>MSGDASSGSPDITGEEQGVAVATGTQPSAPAMATLATAATGTMPEEWKTFFSYYTTVNWSTTDETGKVLFVQGLSPRMNPFLDHLAKMYTGWSGSMEIRFTISGSGVFGGKLAAVMVPPGIGTEGGTSLLQFPHVLVDARQTEPVIFNIPDIRTVLWHDMHDTLTAHLVILVYNDLLNPYQNTTTGTSCTVTVETRGGTDFEFHLLKPPSRKMIFGADPSRLIPKKSMFWEGNRLPGEFKGFSIKPLVFQANRHFDCKRQTFGWSTPEHAGVKLNIQRQNLDTEDKTDIGVHLVTGLKTIKSQVPDGWPDYYGRNIILANTTASFGEVSEAMLGTVVPYRVSGK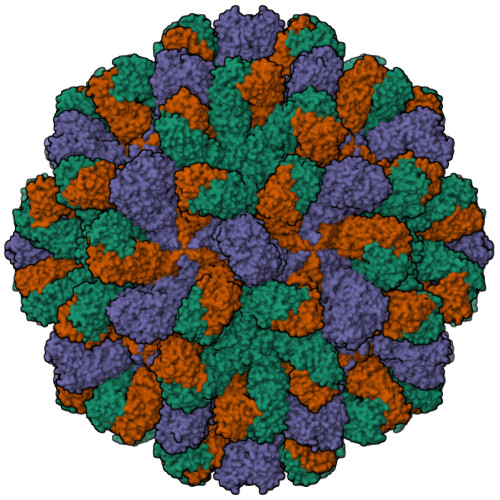LEWRHLPEIAFANGTAKNSTIVCGKYLTGNFYVGGNFTQQGNVVVYPAFWTSKHGDTKCIGEDEDMVKRIDVLPQAQTTGGNYPIYYVTEFPAAYLPAPRVYNSQLLWTSRLLAQDVYDIGPEALAVFKIKDSAGNWFDIGISCEGFSFVGAPTLPFSSLQFPLEASYVGMASAYNKLQHNIAGTSVTL[3x]> MLSPPRRKAFKKWTPPRSPFNLVQETLFHDPWKLLIATIFLNRTSGKMAIPVLWKFLEKYPSAEVARTADWR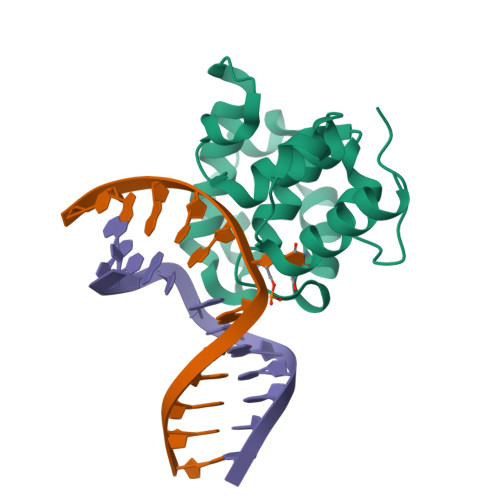DVSELLKPLGLYDLRAKTIVKFSDEYLTKQWKYPIELHGIGKYGNDSYRIFCVNEWKQVHPEAHKLNKYHDWLWENHHHHHHH>[4x]GAMAMNNPLEFKWLEDFLSLMELGNFSAAAKARFVTQSAFSRRIQALEVWIGVPLFDRTSYPITLTEHGQKFVPYAENLLNQVKVTKEDFAQASLKTDHTVRIVCLHTLAVNLLPKLFLQSAEALSHLNLSVTPSVLGIDAHFQMLEDHSTDLLFTYNISAMRPSLSLEDKLEKCVIHSEKVVPVVAPRLLESLKA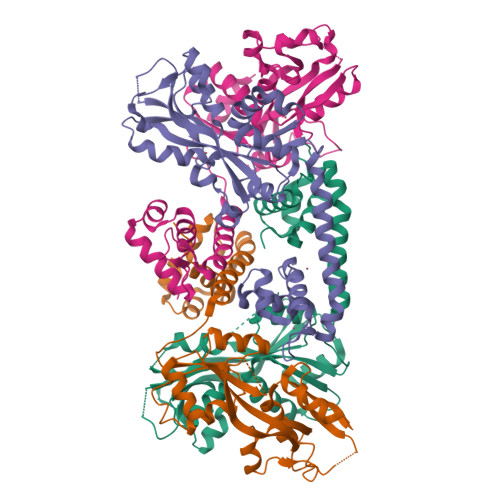DQTIPYLSYSEHTFLSKVVEPVLKTLPLTLKPVFETTLSESLVKMAIGGAGVAWVPMHVIEEELAQHRLVIAFEEQKEWQIPIDILCYRSTTNHRAAVDQFWQEIDKS>VSHFKNCADKQLSDDKPLQCKIRNLQVDGNMPKVKEYMNCAFESSGWAKDGGKKLDTSKVAQDMVPY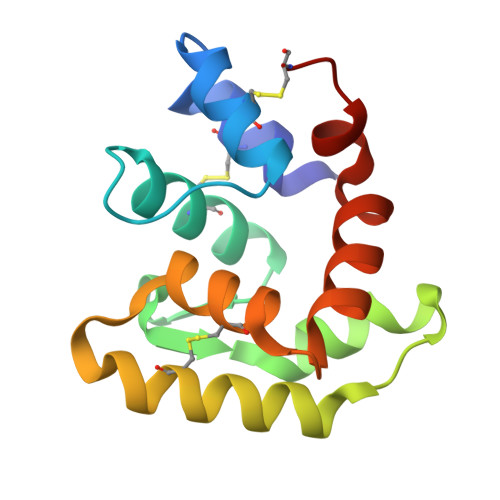GFNIKTELDEVTKECETEFGAEISSIDYLACLLIDEKTKTQFKTMLMMKEADFFKQNLCN[2x]>MGAHASVIKPEMKIKLRMEGAVNGHKFVIEGEGIGKPYEGTQTL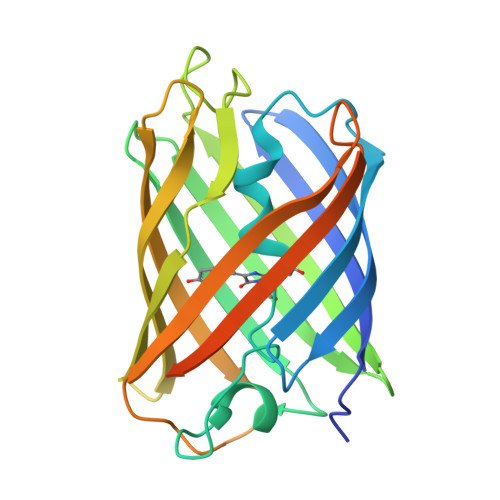DLTVEEGAPLPFSYDILTPAFEYGNRAFTKYPEDIPDYFKQAFPEGYSWERSMTYEDQGICIATSDITMEGDCFFYEIRFDGTNFPPNGPVMQKKTLKWEPSTDKMYVEDGVLKGDVEMALLLEGGGHYRCDFKTTYKAKKDVRLPDAHEVDYRIEILSHDKDYNKVRLYEHAEARYSGGGSGGGASGKPIPNPLLGLDSTHHHHHH[4x]>[4x]ASMTGGQQMGRGSEFMGQSHTHDHHHDGYQAPPEDIALRVKALESLLIEKGLVDPAAMDLVVQTYEHKVGPRNGAKVVAKA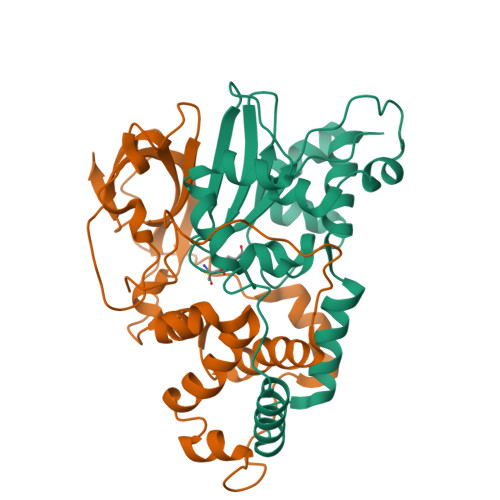WVDPAYKARLLADGTAGIAELGFSGVQGEDMVILENTPAVHNVFVCTLCSCYPWPTLGLPPAWYKAAPYRSRMVSDPRGVLAEFGLVIPANKEIRVWDTTAELRYMVLPERPAGTEAYSEEQLAELVTRDSMIGTGLPTQPTPSH;>[4x]MNGIHDTGGAHGYGPVYREPNEPVFRYDWEKTVMSLLPALLANGNFNLDEFRHSIERMGPAHYLEGTYYELWLHVFENLLVEKGVLTATEVATGKAASGKTATPVLTPAIVDGLLSTGASAAREEGARARFAVGDKVRVLNKNPVGHTRMPRYTRGKVGTVVIDHGVFVTPDTAAHGKGEHPQHVYTVSFTSVELWGQDASSPKDTIRVDLWDDYLEPA Herein, we provide high‐resolution structures for an EAL enzyme Bd1971, from the predatory bacterium Bdellovibrio bacteriovorus, which is controlled by a second signaling nucleotide, cAMP. The Bd1971 domain architecture is predicted to consist of an N‐terminal cNMP sensory domain (cyclic nucleotide monophosphate, postulated to bind cAMP or cGMP), a middle linker region, and C‐terminal catalytic EAL barrel. We reveal that regulation of c‐di‐GMP hydrolysis arises from a domain‐swapping of the “regular” cNMP fold, which undergoes significant rearrangements upon binding of stimulus, communicating a series of conformational changes over 40 Å to license a productive state at the EAL dimer interface. C‐di‐GMP turnover was increased ~8‐fold in the presence of cAMP or cGMP, further supporting the proposal that cNMPs are activators of Bd1971.

Our observation of a classical open/productive EAL dimer for Bd1971 led us to investigate competency for c‐di‐GMP binding at the active site. Crystals of Bd1971 (grown using cAMP ligand) were soaked in solutions supplemented with c‐di‐GMP and Ca2+ (included to prevent substrate turnover). Clear electron density was observed for c‐di‐GMP at both dimer active sites, bound in the expected extended conformation (determined to 2.83 Å resolution, structure in Fig 3E). In comparison with our multiple structures with an empty EAL active site, there are no gross changes upon binding substrate; this is distinct from MorA, whose H‐helix (mapping to the Bd1971 interdomain linker helix) and associated GGDEF domain undergo a 20˚ rotation when c‐di‐GMP binds (Phippen et al, 2014). Smaller, local changes upon binding are limited to the metal‐binding pocket (which like other EAL domains, binds one metal in the empty state and two metals in the substrate complex), and residues which undergo rotameric changes to accommodate c‐di‐GMP (Arg330 shifts to relieve a clash with the nucleotide base and ribose, Arg182 and Tyr385 move inward to interact with base and phosphate, respectively). Structure of the cyclic‐di‐GMP bound complex of Bd1971 (ligand C represented in yellow, bound Ca2+ ions as green spheres). Residues R182, R330, and Y385 display the largest shift between the apoenzyme (tan) and bound (blue) states, R182 complexing the cyclic‐di‐GMP phosphate, and Y385 stacking with a guanine base. The configuration of the active site residues of Bd1971 is similar to other (active) EAL structures, further indicating that this form represents the active state of the Bd1971 EAL domain; hence, we instigated further study into how the novel domain structure (with a stimulus‐sensing cNMP domain) could switch EAL activation states.

>AQSVDIHKDQIIFSEGDAGDCAYIIEKGRVLIYLTKDKEEIPLTILGEGEIFGEMALIDNQNRSASVRALEDVRLAIVTKQQVLERVSTADKVVQLLMRVLLKRLRRKNIGGPGGSRISEVEFDNSGAGDDGTQSALDQIKLENQIFQAFQNKEFELFYQPIVNLKNKTITGCEALLRWNSPQHGLVSPNLFIDIIENSSMVIPIGHWIINQALKDLRTIQDQLRLNKKERMADDFMMSINISGRQFTHSDFVNNLEDLREKHDLHTQNIKLEMTERIMMDGAIAIDALNQCRSLGYAISIDDFGTGFSGLQYLTQMPISFLKIDRSFVMKILSDPKSKAVVSSIIHLAHAMDIEVIAEGIEHHEEALVLETLGARFGQGYLFSKPVDLGRFLKLIKL[2x]> MAEYKDNLLGEANSFLEVLEQVSHLAPLDKPVLIIGERGTGKELIASRLHYLSSRWQGPFISLNCAALNENLLDSELFGHEAGAFTGAQKRHPGRFERADGGTLFLD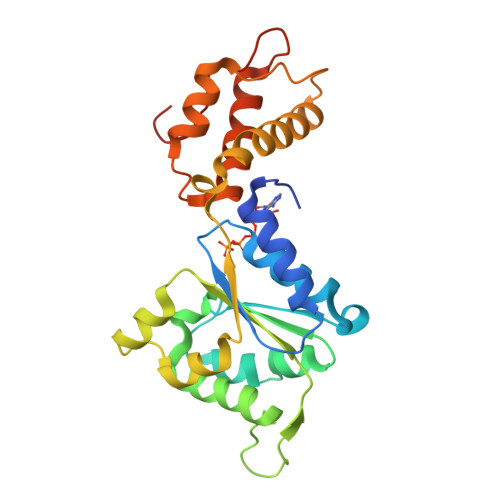ELATAPMMVQEKLLRVIEYGELERVGGSQPLQVNVRLVCATNADLPAMVNEGTFRADLLDRLAFDVVQLPPLRERESDIMLMAEYFAIQMCREIKLPLFPGFTERARETLLNYRWPGNIRELKNVVERSVYRHGTSDYPLDDIIIDPFKRRPPEDAIA> MPPQLHNGLDFSAKVIQGSLDSLPQEVRKFVEGNAQLCQPEYIHICDGSEEEYGRLLAHMQEEGVIRKLKKYDNCWLALTDPRDVARIESKTVIITQEQRDTVPIPKSGQSQLGRWMSEEDFEKAFNARFPGCMKGRTMYVIPFSMGPLGSPLAKIGIELTDSPYVVASMRIMTRMGTSVLEALGDGEFIKCLHSVGCPLPLKKPLVNNWACNPELTLIAHLPDRREIISFGSGYGGNSLLGKKCFALRIASRLAKEEGWLAEHMLILGITNPEGKKKYLAAAFPSACGKTNLAMMNPTLPGWKVECVGDDIAWMKFDAQGNLRAINPENGFFGVAPGTSVKTNPNAIKTIQKNTIFTNVAETSDGGVYWEGIDE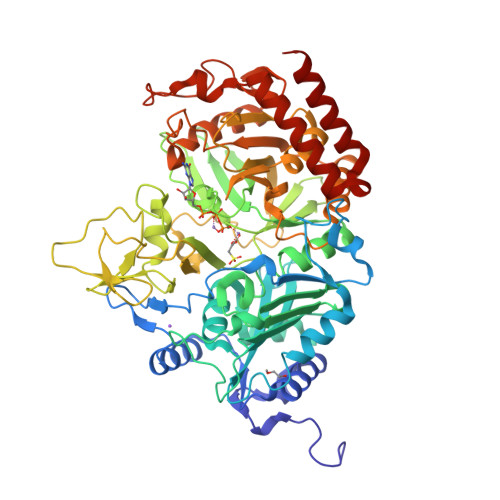PLAPGVTITSWKNKEWRPQDEEPCAHPNSRFCTPASQCPIIDPAWESPEGVPIEGIIFGGRRPAGVPLVYEALSWQHGVFVGAAMRSEGGGIMHDPFAMRPFFGYNFGKYLAHWLSMAHRPAAKLPKIFHVNWFRKDKNGKFLWPGFGENSRVLEWMFGRIEGEDSAKLTPIGYVPKEDALNLKGLGDVNVEELFGISKEFWEKEVEEIDKYLEDQVNADLPYEIERELRALKQRISQM> AGAGAAGUU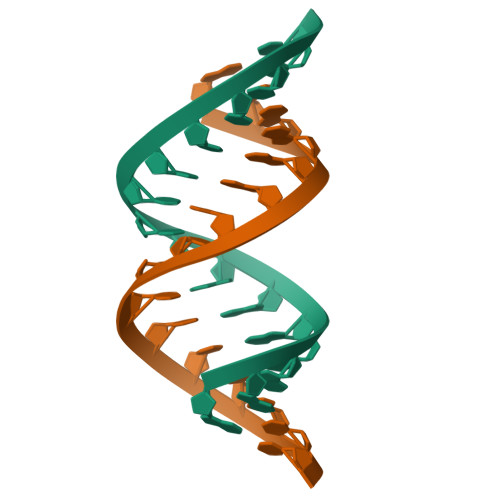CUUCUCU>[2x]HHHHHHTDRFTRLLGIQQPIIQAPMLGVSTPALAAAVSNAGGLGSIAITGSAAEKGRALIREVRGLTDKPFNVNLFCHRPGQADPARERAWLDYLKPLFAEFGAEPPVRLKNIYLSFLEDPTLLPMLLEERPAAVSFHFGAPPRDQVRALQAVGIRVLVCATTPEEAALVEAAGADAVVAQGIEAGGCRGVFEPERGDA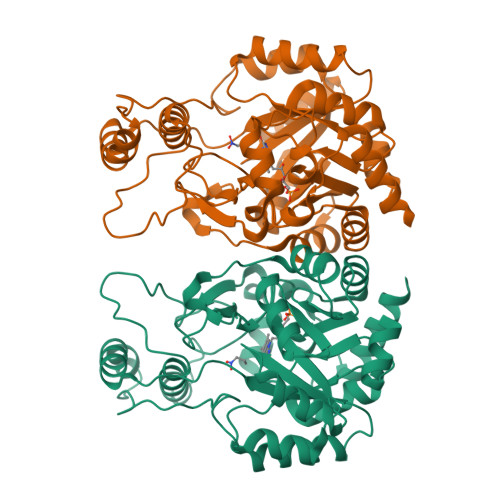AIGTLALVRLLAARGSLPVVAAGGIMDGRGIRAALELGASAVQMGTAFVLCPESSANAAYREALKGPRAARTALTVTMSGRSARGLPNRMFFDAAAPGVPPLPDYPFVYDATKALQTAALARGNHDFAAQWAGQGAALARELPAAELLRTLVEELRG6-[({(2S)-1-amino-4-[(6-amino-4-methylpyridin-2-yl)methoxy]butan-2-yl}oxy)methyl]-4-methylpyridin-2-amine | C18 H27 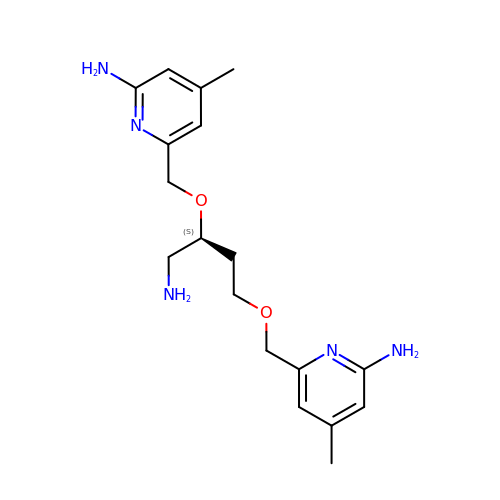N5 O2 | ZLWWYKPNQBCOKF-INIZCTEOSA-N>[2x]SQDIVDFSQHPWKAPGPNDLRSPCPGLNTLANHGFLPRNGRNITIPMIVQAGFDGYNVQPDILILAAKVGLLTSPEPDTFTLDDLKLHGTIEHDASLSREDFALGDNLHFNEAIFNTLANSNPGSDVYNITSAGQVLKDRLADSLARNPNVTNTGKEFTIRTLESAFYLSVMGNATTGEAPKNFVQIFFREERLPIEEGWKRSTTPITSDTLNPIAGQISEASNWKPNPDQCPWIVLSPNL

Unspecific peroxygenases (UPOs) are a class of heme‐thiolate oxygenases from fungi that have similar catalytic scope to P450s, but are dependent only upon hydrogen peroxide (H2O2) as the external oxidant. A recent survey by Faiza and co‐workers explored the diversity of UPOs within sequence databases and was able to identify two major groups of enzymes: ‘long’ UPOs (Group I), typified by AaeUPO, of approximately 45 kDa molecular weight, and ‘short’ UPOs (Group II), typified by the enzyme from Marasmius rotula (MroUPO), which are of approximately 29 kDa. In this study, we have cloned the gene encoding an ‘artificial’ short UPO (artUPO) close in sequence to MroUPO, and expressed it in both Pichia pastoris and E. coli. In addition to their overall similarities in fold, artUPO, MroUPO and HspUPO feature both a glutamic acid and histidine residue (E164 and H93 in artUPO) that forms the catalytic acid‐base pair, in common with CPO and in contrast to the Glu‐Arg dyad found in AaeUPO.

The structure of the artUPO expressed in E. coli was also determined to see if there were any significant differences that may result from a lack of in vivo glycosylation. artUPObact crystals were obtained in the P212121 space group and again featured two molecules in the asymmetric unit, forming a dimer that was again connected by a disulfide bridge between residues C232. The monomers superimposed with an rmsd of 0.26 A over 232 C alpha atoms, reflective of their very high structural similarity. Few obvious differences could be discerned between the structures of artUPOyeast and artUPObact, except that the N‐terminal residues D6, F7 and S8 could be modelled in the latter, but not the former, and there was of course no glycosylation on asparagine sites N42, N129, N150 and N174 in the bacterially expressed enzyme. We studied both the melting temperatures (T m) and onset of aggregation temperatures of artUPOyeast and artUPObact using nano differential scanning fluorimetry (nano‐DSF). artUPObact gave a simple profile with a calculated T m of 47.8 °C, but artUPOyeast gave a more complex two‐phase profile from which the first T m was determined to be 45.5 °C, but the second value could not be determined. The results clearly show that the onset of aggregation for artUPObact of approximately 59 °C is significantly lower than that for artUPOyeast. This lower stability may be a direct consequence of the lack of glycosylation and was indeed manifested in visible precipitation of artUPObact in biotransformation reactions (vide infra). Despite this difference in peroxidase activity, the catalytic efficiency of peroxygenase activity toward NBD of artUPOyeast and artUPObact was more or less equivalent. The enzyme was challenged with para‐methylthioanisole 23 under similar reaction conditions to those used for artUPOyeast, giving a 65 % conversion to sulfoxide after 2 h.>MSQTHKHAIPANIADRCLINPEQYETKYKQSINDPDTFWGEQGKILDWITPYQKVKNTSFAPGNVSIKWYEDGTLNLAANCLDRHLQENGDRTAIIWEGDDTSQSKHISYRELHRDVCRFANTLLDLGIKKGDVVAIYMPMVPEAAVAMLACARIGAVHSVIFGGFSPEAVAGRIIDSSSRLVITADEGVRAGRSIPLKKN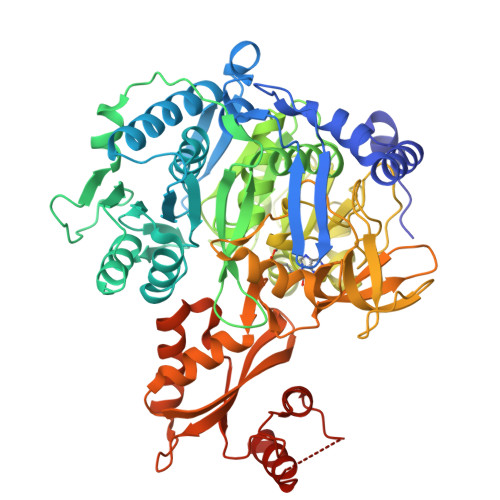VDDALKNPNVTSVEHVIVLKRTGSDIDWQEGRDLWWRDLIEKASPEHQPEAMNAEDPLFILYTSGSTGKPKGVLHTTGGYLVYAATTFKYVFDYHPGDIYWCTADVGWVTGHSYLLYGPLACGATTLMFEGVPNWPTPARMCQVVDKHQVNILYTAPTAIRALMAEGDKAIEGTDRSSLRILGSVGEPINPEAWEWYWKKIGKEKCPVVDTWWQTETGGFMITPLPGAIELKAGSATRPFFGVQPALVDNEGHPQEGATEGNLVITDSWPGQARTLFGDHERFEQTYFSTFKNMYFSGDGARRDEDGYYWITGRVDDVLNVSGHRLGTAEIESALVAHPKIAEAAVVGIPHAIKGQAIYAYVTLNHGEEPSPELYAEVRNWVEKEIGPLATPDVLHWTDSLPKTRSGKIMRRILRKIAAGDTSNLGDTSTLADPGVVEKLLEEKQAIAMPS[2x]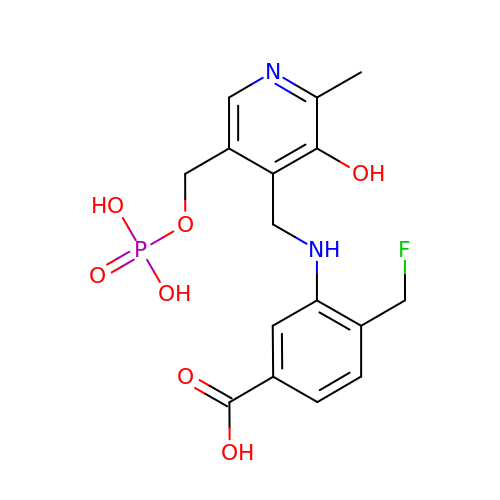(4~{R})-4-(fluoranylmethyl)-3-[[2-methyl-3-oxidanyl-5-(phosphonooxymethyl)pyridin-4-yl]methylamino]cyclohexene-1-carboxylic acid | C16 H18 F N2 O7 P | MGRVCHMHEIIJND-UHFFFAOYSA-N The Papain-like protease (PLpro) is a domain of a multi-functional, non-structural protein 3 of coronaviruses. PLpro cleaves viral polyproteins and posttranslational conjugates with poly-ubiquitin and protective ISG15, composed of two ubiquitin-like (UBL) domains. PolyUb and ISG15 have common other structural features: ISG15 comprises two Ub-like (UBL) domains and mimics a head-to-tail linked di-ubiquitin (Ub2). While K48-linked Ub2 (K48-Ub2) and ISG15 are similar both in sequence and fold, the topologies of how the two domains are linked are distinct.

We additionally determined structures of the free hISG15 and K48-Ub2 to 2.15 and 1.25 Å resolution, respectively. The bound and free hISG15 conformations are similar with a root-mean-square deviation (rmsd) for Cα atoms of 1.34 Å based on the alignment of the C-terminal (proximal) UBL. In ISG15, the two UBL domains are connected through a relatively short, likely more rigid peptide linker (DKCDEP in hISG15), and the C-terminal (proximal) UBL binds to S1 site while the N-terminal (distal) UBL binds to S2 site on PLproCoV-2.

>[6x]SNAGWDLTVKMLAGNEFQVSLSSSMSVSELKAQITQKIGVHAFQQRLAVHPSGVALQDRVPLASQGLGPGSTVLLVVDKCDEPLSILVRNNKGRSSTYEVRLTQTVAHLKQQVSGLEGVQDDLFWLTFEGKPLEDQLPLGEYGLKPLSTVFMNLRLRGG>[2x]MLPKDKLNPPTPSIYLENKRDAFFPPLHQFCTNPKNPVTVIRGLAGALKLDLGLFSTKTLVEANNEHMVEVRTQLLQPADENWDPTGTKKIWRCESNRSHTTIAKYAQYQASSFQESLREENEKRTQHKDHSDNESTSSENSGRRRKGPFKTIKFGTNIDLSDNKKWKLQLHELTKLPAFARVVSAGNLLTHVGHTILGMNTVQLYMKVPGSRTPGHQENNNFCSVNINIGPGDCEWFVVPEDYWGVLNDFCEKNNLNFLMSSWWPNLEDLYEANVPVYRFIQRPGDLVWINAGTVHWVQAVGWCNNIAWNVGPLTACQYKLAVERYEWNKLKSVKSPVPMVHLSWNMARNIKVSDPKLFEMIKYCLLKILKQYQTLREALVAAGKEVIWHGRTNDEPAHYCSICEVEVFNLLFVTNESNTQKTYIVHCHDCARKTSKSLENFVVLEQYKMEDLIQVYDQFTLALSLSSSSAENLYFQ

KDM6A (UTX) and KDM6B (JMJD3) are KDM6 subfamily members that catalyze demethylation of Nϵ-methylated histone 3 lysine 27 (H3K27), a mark important for transcriptional repression. Despite reports stating that UTY(KDM6C) is inactive as a KDM, we demonstrate by biochemical studies, employing MS and NMR, that UTY(KDM6C) is an active KDM. Crystallographic analyses reveal that the UTY(KDM6C) active site is highly conserved with those of KDM6B and KDM6A. UTY(KDM6C) catalyzes demethylation of H3K27 peptides in vitro, analogously to KDM6B and KDM6A, but with reduced activity, due to point substitutions involved in substrate binding.

The first helix in KDM6A and the linker region (residues 886–902 in KDM6A) that connects the helical and JmjC domains are not observed in our current crystal structure of UTY(KDM6C). The UTY(KDM6C) JmjC domain contains 13 β-strands and 10 helices, including the extended and distorted double-stranded β-helix that is characteristic of the 2OG oxygenase superfamily. At the active site, the nature of coordination by the metal binding residues is also well conserved, with metal binding by the Nϵ-imidazole nitrogens of His1093 and His1173 and by the carboxylate of Glu1095. Analysis of the electron density at the active site supports presence of 2OG in the cofactor binding pocket. 2OG coordinates the active site metal in a bidentate manner via its oxalyl group, with a water-ligated coordination site adjacent to the predicted location of the substrate Nϵ-methylated lysine group (as observed in KDM6B and KDM6A enzyme-substrate complexes). Notably, the unusual (within structurally characterized 2OG oxygenases) presence of two cysteinyl residues (Cys1111 and Cys1181) in the 2OG binding pocket is observed in UTY(KDM6C) as in other KDM6 subfamily members. In each of the KDM6 subfamily members' zinc-binding domains, the Zn(II) is coordinated by four cysteines, Cys1278, Cys1281, Cys1305, and Cys1308, in UTY(KDM6C). Comparison of the structures reveals that the Fe(II)/2OG binding sites are highly conserved in all human KDM6 members. Superposition of the three structures implies that most of the hydrogen-bonding interactions in KDM6A/B substrate binding probably occur in UTY(KDM6C). Notably, however, one residue, located in the loop between the JmjC and helical domains and which in KDM6A (Ile1267) and KDM6B (Ile1511) appears to form hydrophobic interactions with Ala25 of the H3K27Me3 substrate, is substituted for a prolyl residue (Pro1214) in UTY(KDM6C) (see below).> MSMYTTAQLLAANEQKFKFDPLFLRLF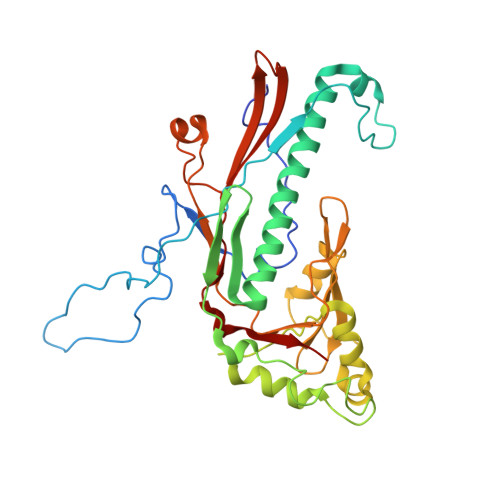FRESYPFTTEKVYLSQIPGLVNMALYVSPIVSGEVIRSRGGSTSEFTPGYVKPKHEVNPQMTLRRLPDEDPQNLADPAYRRRRIIMQNMRDEELAIAQVEEMQAVSAVLKGKYTMTGEAFDPVEVDMGRSEENNITQSGGTEWSKRDKSTYDPTDDIEAYALNASGVVNIIVFDPKGWALFRSFKAVKEKLDTRRGSNSELETAVKDLGKAVSYKGMYGDVAIVVYSGQYVENGVKKNFLPDNTMVLGNTQARGLRTYGCIQDADAQREGINASARYPKNWVTTGDPAREFTMIQSAPLMLLADPDEFVSVQLA> GSTGGVQTVTLIPGDGIGPEISAAVMKIFDAAKAPIQWEERNVTAIQGPGGKWMIPSEAKESMDKNKMGLKGPLKTPIAAGHPSMNLLLRKTFDLYANVRPCVSIEGYKTPYTDVNIVTIRENTEGEYSGIEHVIVDGVVQSIKLITEGASKRIAEFAFEYARNNHRSNVTAVHKANIMRMSDGLFLQKCREVAESCKDIKFNEMYLDTVCLNMV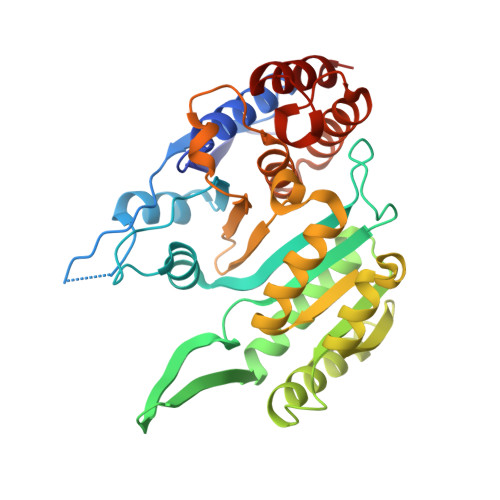QDPSQFDVLVMPNLYGDILSDLCAGLIGGLGVTPSGNIGANGVAIFESVHGTAPDIAGKDMANPTALLLSAVMMLRHMGLFDHAARIEAACFATIKDGKSLTKDLGGNAKCSDFTEEICRRVKDLD>[2x]GAMKKKSLTELISDLKGNENVVNWHEIEPREAKTRPMPESIDERIKAALSKRGIDELYTHQYSAFQYVQKGESIVTVTPTASGKTLCYNLPVLQSIAQDETNRALYLFPTKALAQDQKSELNEIIDEMGIDIKSFTYDGDTSPAIRQKVRKAGHIVITNPDMLHSAILPHHTKWVSLFENLKYIVIDELHTYRGVFGSHVANVIRRLKRICRFYGSDPVFICTSATIANPKELGEQLTGKPMRLVDDNGAPSGRKHFVFYNPPIVNKPLNIRRSATAEVNELAKEFLKNKVQTIVFARSRVRVEIILSHIQELVKKEIGTKSIRGYRGGYLPKERREIERGLREGDILGV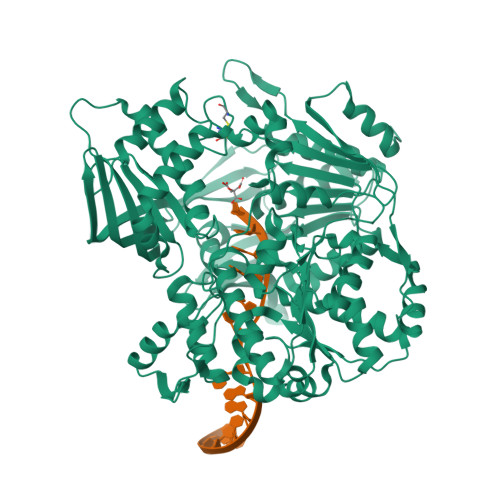VSTNALELGVDIGQLQVCVMTGYPGSVASAWQQAGRAGRRHGESLIIMVANSTPIDQYIVRHPEYFFNRSPESARINPENLIILVDHLKCAAYELPFRADEEFGAMEVSDILEYLQEEAVLHRNGERYHWASESFPASNISLRSASQENVVIVDQSDIANVRIIGEMDRFSAMTLLHDEAIYLHEGVQYQVEKLDWDHKKAYVRKVDVEYYTDANLAVQLKVLEIDKTKEKSRTSLHYGDVTVNALPTIFKKIKMTTFENIGSGPIHLPEEELHTSAAWLEIKTADEDIGEKTLEQLLLGISNVLQHIVPVYIMCDRNDVHVVSQIKAAHTGLPTIFLYDHYPGGIGLAEEVFKRFSDINEAAKQLITHCPCHDGCPSCIGTEIEGIKAKERILQLLDQMS3-HYDROXYPYRUVIC ACID | C3 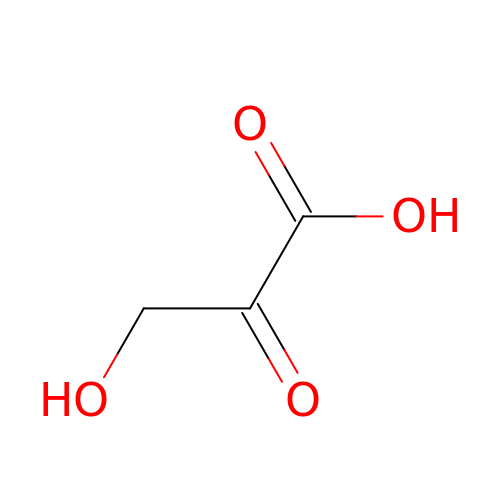H4 O4 | HHDDCCUIIUWNGJ-UHFFFAOYSA-N>AEVPLPQLRAYTVDASWLQPMAPLQIADHTWQIGTEDLTALLVQTPDGAVLLDGGMPQMASHLLDNMKARGVTPRDLRLILLSHAHADHAGPVAELKRRTGAKVAANAESAVLLARGGSDDLHFGDGITYPPANADRIVMDGEVITVGGIVFTAHFMAGHTPGSTAWTWTDTRNGKPVR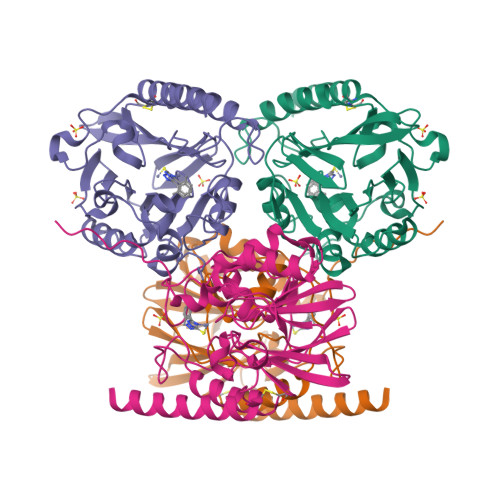IAYADSLSAPGYQLQGNPRYPHLIEDYRRSFATVRALPCDVLLTPHPGASNWDYAAGARAGAKALTCKAYADAAEQKFDGQLAKETAGAR[2x]{(3R,5R,6S)-5-(3-chlorophenyl)-6-(4-chlorophenyl)-1-[(1S)-1-(6-cyclopropylpyridin-2-yl)propyl]-3-methyl-2-oxopiperidin-3-yl}acetic acid | C31 H32 Cl2 N2 O3 | 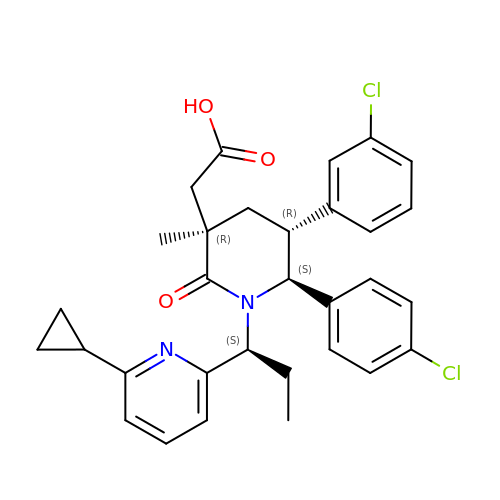QHQNRLZCHQCYRC-IEPITWRRSA-N RecF is a multifunctional protein involved in recombinant DNA repair, homologous genetic recombination, and DNA replication. Similar to RecR and RecO, RecF is a recombination mediator protein (RMP) in the RecFOR pathway for ssDNA gap repair. RecF contains the conserved Walker A motif, Walker B motif and signature motif of ABC-ATPase that exhibits ATP-dependent dimerization; additionally, the signature motif residues interact with the ATP bound to the opposite molecule. To gain insight into the mechanism of ABC-ATPase RecF, we solved the crystal structures of TTERecF, TTERecF-ATP, and TTERecF-ATPɤS.

The structure of TTERecF-ATPɤS is also a dimer, that is completely different from the dimer of TTERecF-ATP and is thus another conformation of TTERecF. In the TTERecF-ATPɤS structure, domain I of the two monomers interacted, whereas their respective domain II structures were located far from each another. The dimer contact surface was 2613 Å2, which was 7.7% of the dimer total surface area (33774 Å2). The two monomers of TTERecF-ATPɤS were dissimilar; one monomer consisted of TTERecF-ATPɤS and the other consisted of TTERecF only. One monomer structure (ATPɤS binding) was nearly similar to one monomer of TTERecF-ATP dimer, including the active site conformation of the Walker A motif, Walker B motif, and signature motif. The Cα atoms of these two structures can be superimposed with an r.m.s.d of 0.807 Å. The other monomer structure (no ATPɤS binding) was similar to that of the free TTERecF; the r.m.s.d of the superimposed Cα atoms was 1.121 Å. According to the structure and interface of electrostatic potential, the interacting amino acids were mainly located in the RecF helix αF from the structure of TTERecF-ATPɤS. Thus, we were sure that the RecF helix αF is the interface of the RecF-ATPrS dimer. In addition, the DNA binding affinities of the TTERecF-ATPɤS dimer for 21-mer ssDNA and dsDNA were 466 nM and 381 nM, which did not significantly differ from those of the native TTERecF. The structural and biochemical data showed that the TTERecF-ATPɤS dimer cannot stably bind with DNA.

>HHHSQDPMYLKEIFVDNFRNLKKQKLEFCEGVNLIYGLNAQGKSNLLEAIRLLSMGRSFRGSKMSELVKFDEEYFYVRGLVRSADFYEKKIEFGYKVNGNKVIKVNGNKLKSTGEILGHFLTVIFSPEDIEIIKEGPSRRRKYLDACISVIDKNYFFDLLQYNKTLSNRNSLLKKIKEEGKGEDLLEIFDEKLAEYGARIIKVRNNYLEKLKNSMSKFLMEISNEKLEIIYLNSAGVKEVHEENLIREKLKNRLTKSLTLDLKYLSTQVGPHREDFKILINGYDSRVYSSQGQKRTAALCLKLSELEILEEETGEKPVLLLDDVMSELDDNRKKYILKKLEGFQSFITHTSKSDVEGDCCFKIYDGIVDKLA[2x]>[2x]GSHHHHHHGSFSEDVLGWRESFDLLLNSKNGVAAFHAFLKTEFSEENLEFWLA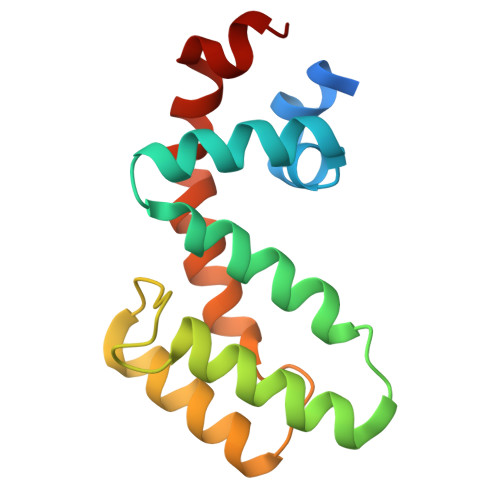CEEFKKIRSATKLASRAHHIFDEYIRSEAPKEVNIDHETRELTKTNLQAATTSCFDVAQGKTRTLMEKDSYPRFLKSPAYRDLA>MAHHHHHHMSKPKVGINGFGRIGRLVLRAAVEKDTVDVVAVNDPFINIDYMVYMFKYDSTHGRFKGSVSAEGGKLIVTNGKTTHHISVHNSKDPAEIPWGVDGAEYVVESTGVFTTTDKASAHLKGGAKKVII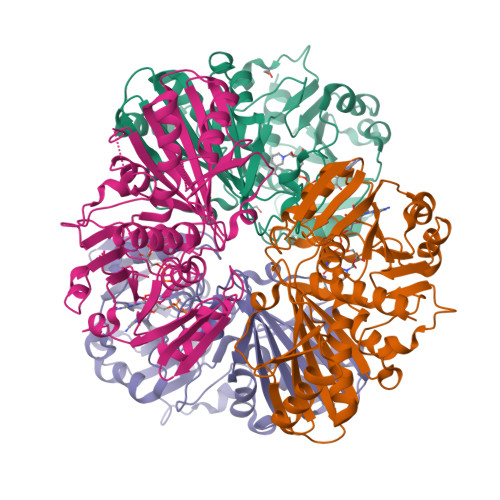SAPSADAPMFVMGVNNDTYDKANNHIISNASCTTNCLAPLAKVIHDKFGIIEGLMTTVHATTATQKTVDGPSGKLWRDGRGAGQNIIPASTGAAKAVGKVIPDLNGKLTGMAFRVPTPDVSVVDLTCRLQKGATMDEIKAAVKEAANGPMKGILEYTEDQVVSTDFTGDTHSSIFDALACISLNPNFVKLIAWYDNEYGYSNRVVDLISYIASR[8x]> 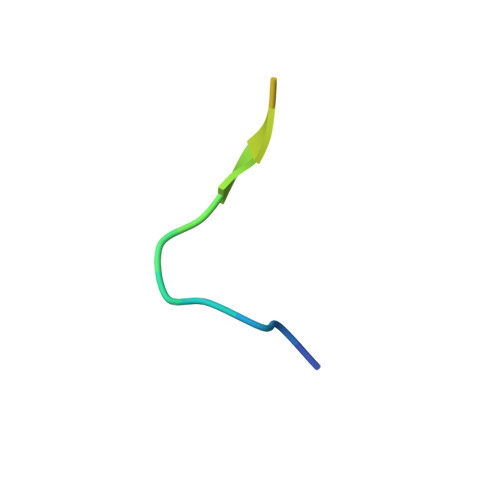YSAYPDSVPMMSGSGSK2-methoxyethyl (2E)-3-phenylprop-2-en-1-yl 2,6-dimethyl-4-(3-nitrophenyl)pyridine-3,5-dicarboxylate 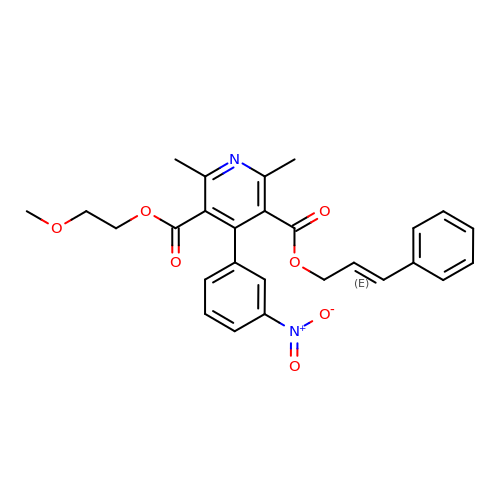| C27 H26 N2 O7 | HUTPFIMQINDZDT-DHZHZOJOSA-N> QIIGTVPGVEVGDEFQYRMELNLLGIHRPSQSGIDYMKDDGGELVATSIVSSGGYNDVLDNSDVLIYTGQGGNVGKKKNNEPPKDQQLVTGNLALKNSINKKNPV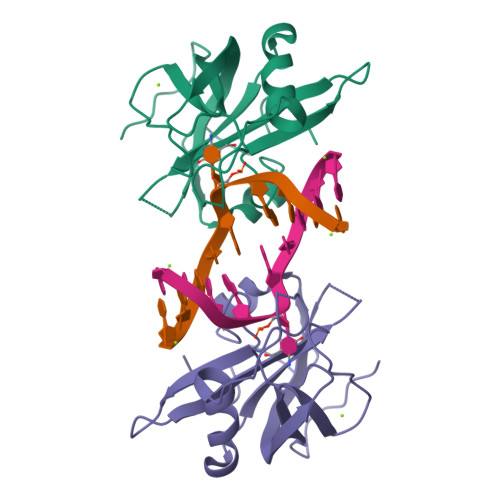RVIRGIKNTTLQSSVVAKNYVYDGLYLVEEYWEETGSHGKLVFKFKLRRIPGQPELPWKEVA(5S)-5-(dioxidanyl)-9-methyl-7H-purine-2,6,8-trione | C6 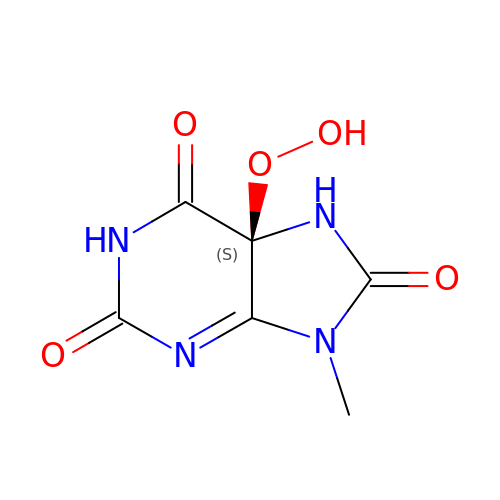H6 N4 O5 | JQXTWGOGXIASQD-LURJTMIESA-N> SSNDNIELVDFQNIMFYGDAEVGDNQQPFTFILDTGSANLWVPSVKCTTAGCLTKHLYDSSKSRTYEKDGTKVEMNYVSGTVSGFFSKDLVTVGNLSLPYKFIEVIDTNGFEPTYTASTFDGILGLGWKDLSIGSVDPIVVELKNQNKIENALFTFYLPVHDKHTGFLTIGGIEERFYEGPLTYEKLNHDLYWQITLDAHVGNIMLEKANC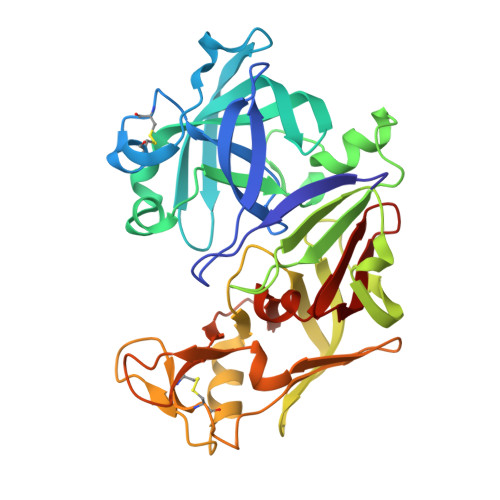IVDSGTSAITVPTDFLNKMLQNLDVIKVPFLPFYVTLCNNSKLPTFEFTSENGKYTLEPEYYLQHIEDVGPGLCMLNIIGLDFPVPTFILGDPFMRKYFTVFDYDNHSVGIALAKKNL Para-hydroxybenzoate hydroxylase (PHBH) is a group A flavoprotein monooxygenase that hydroxylates p-hydroxybenzoate to protocatechuate (PCA). Among proteins in this clade, Xylophilus ampelinus PobA (XaPobA) preferred PCA as a substrate and is the first known natural PCA 5-hydroxylase (PCAH). The overall structure of XaPobA comprised a homodimer, with each unit binding an oxidized form of FAD in its active site. The XaPobA monomer consisted of FAD-(amino acids 1–73, 88–198, and 267–391)- and substrate (amino acids 74–87 and 199–266)- binding domains.

In contrast, XaPobA replaced the Thr347 residue with Cys347, which has a side chain that does not interact with Thr294. The kcat value for PCA was 20-fold lower for the XaPobA C347T mutant that mimicked PaPobA, and 2-fold higher for pHBA, compared with WT XaPobA. Pre-steady state FAD reduction by the C347T mutant in the presence of PCA proceeded at a 30-fold lower rate (kred = 6.5 ± 0.7 × 10−1 s−1) than WT XaPobA. These results indicated that Cys347 is involved in the ability of XaPobA to discriminate PCA. We also determined the ligand-free crystal structure of the C347T mutant at a resolution of 2.06 Å. The Thr347 residue formed a hydrogen bond with Thr294 and fixed the peptide bond in a conformation similar to those of XaPobA + PCA and PaPobA. Taken together, these results indicated that Cys/Thr347, located distal to the active center, plays a role in fine-tuning the position of the Thr294-Gly295 region that fits PCA to the hydrophobic cavity, and regulates the substrate preference of PobA.

>[2x]MQLSHHHHHHSSGLVPRGSHMRTQVGIVGAGPAGLMLAHLLRREGIDAVVIERAAREHVRTRLRAGVLEQGTVEMLREAGVGGRIDAVGMEMHAIDFRFGGRSHRLDFHEASGGRRAWVYPQHEVVTDLMSACDAGDVPILYEAPVERIEGLEDDRARIVFGQDGAAGEITCDFVAGCDGFRGVSRGSMPAGIARGYDRIYPFGWLGILADAPPASPDVTWGCSDRGFAMMSMRSPTVTRLYLQCEPDEDPDAWSDDRIWSELHRRLDVEGMPSLREGPIRDKGVTAMRSFLSEPMQHGRLFLAGDAAHIVPPTGAKGLNSAMADIKVLAAALVDHYRHGRSDRLATYSERCLRRMWLVQRFSAALTTMVHQFPGQNEFVRRLQRADLDYMTGTHAGRLQFAENFTGLPIE> MARLNITFSPQAFEDYKYFQQNDKKMVKKINELLKSIDRNGALEGIGKPEKLKSNLTGYYSRRINHEHRLVYTVDDNHIKIAS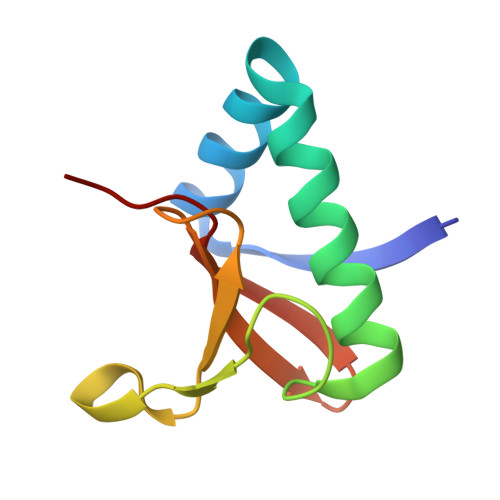CKYHY>GPNPYERGPDPTEDSIEAIRGPFSVATERVSSFASGFGGGTIYYPRETDEGTFGAVAVAPGF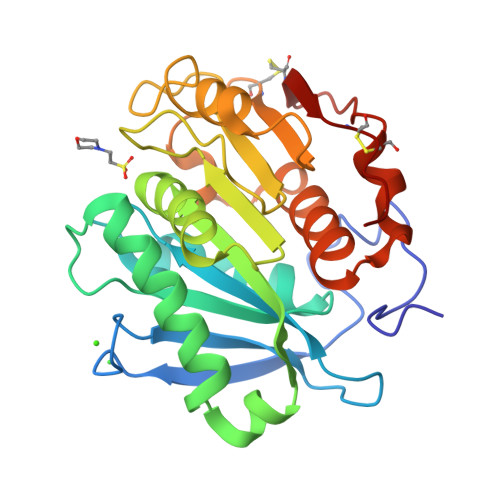TASQGSMSWYGERVASHGFIVFTIDTNTRLDAPGQRGRQLLAALDYLVERSDRKVRERLDPNRLAVMGHAMGGGGSLEATVMRPSLKASIPLTPWHLDKTWGQVQVPTFIIGAELDTIAPVSTHAKPFYESLPSSLPKAYMELCGATHFAPNIPNTTIAKYVISWLKRFVDEDTRYSQFLCPNPTDRAICEYRSTCPYKLN[2x]> KAVVPGPAEHPLQYNYTFWYSRRTPGRPTSSQSYEQNIKQIGTFASVEQF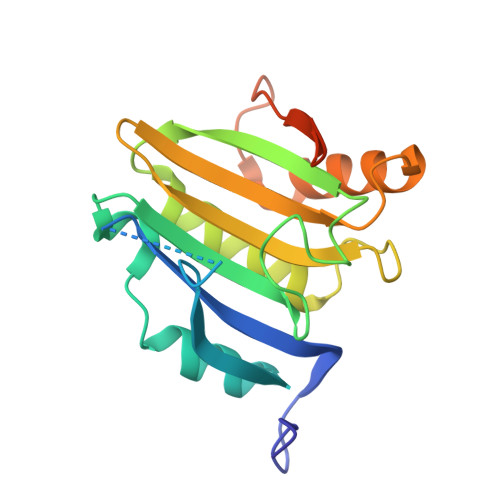WRFYSHMVRPGDLTGHSDFHLFKEGIKPMWEDDANKNGGKWIIRLRKGLASRCWENLILAMLGEQFMVGEEICGAVVSVRFQEDIISIWNKTASDQATTARIRDTLRRVLNLPPNTIMEYKTHTDSIKMPGRLGPQRLLF>[2x]VRSTPPASAGRSTPPALAGHSTPPALAGHSTLCGRPVAGDRALIMAIVNRTPDSFYDKGATFSDAAARDAVHRAVADGADVIDVGGVKAGPGERVDVDTEITRLVPFIEWLRGAYPDQLISVDTWRAQVAKAACAAGADLINDTWGGVDPAMPEVAAEFGAGLVCAHTGGALPRTRPFRVSYGTTTRGVVDAVISQVTA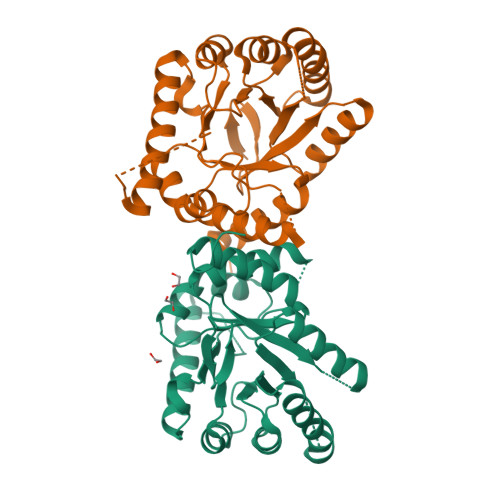AAERAVAAGVAREKVLIDPAHDFGKNTFHGLLLLRHVADLVMTGWPVLMALSNKDVVGETLGVDLTERLEGTLAATALAAAAGARMFRVHEVAATRRVLEMVASIQGVRPPTRTVRGLA S-[2-({N-[(2S)-2-hydroxy-3,3-dimethyl-4-(phosphonooxy)butanoyl]-beta-alanyl}amino)ethyl] hexadecanethioate | C27 H53 N2 O8 P S | 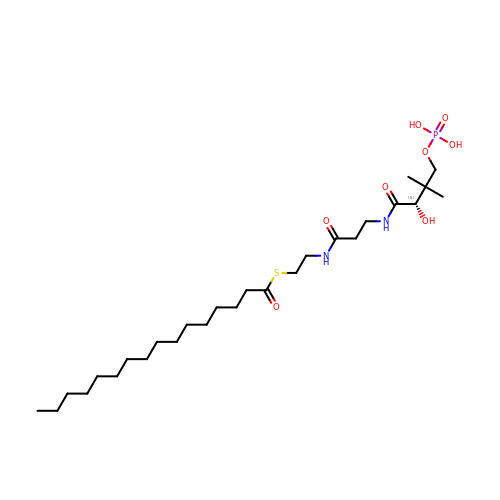JSWBEHRITPIXLC-RUZDIDTESA-N>GPLGSMAGDSEQTLQNHQQPNGGEPFLIGVSGGTASGKSSVCAKIVQLLGQNEVDYRQKQVVILSQDSFYRVLTSEQKAKALKGQFNFDHPDAFDNELILKTLKEITEGKTVQIPVYDFVSHSRKEETVTVYPADVVLFEGILAFYSQEVRDLFQMKLFVDTDADTRLSRRVLRDISERGRDLEQILSQYITFVKPAFEEFCLPTKKYADVIIP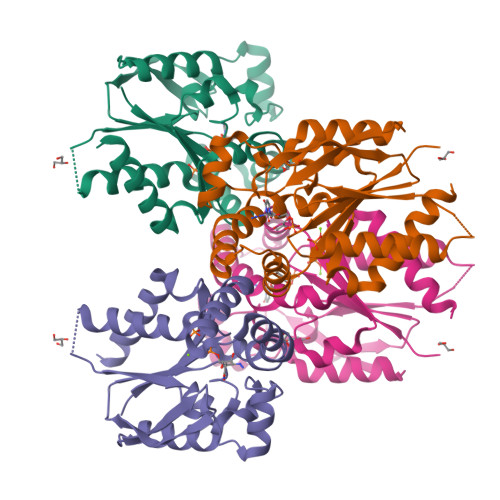RGADNLVAINLIVQHIQDILNGGPSKRQTNGCLNGYTPSRK[2x]>[2x]APRKFFVGGNWKMNGDKKSLGELIHTLNGAKLSADT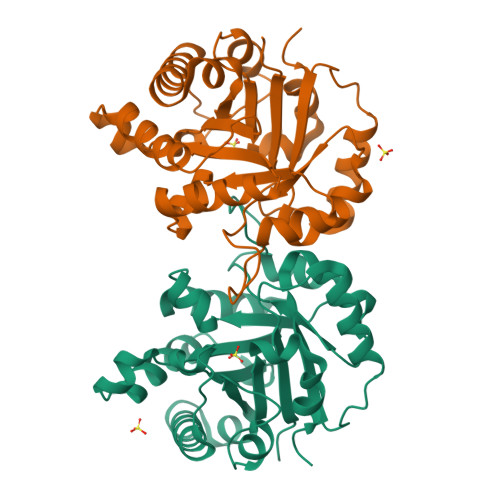EVVCGAPSIYLDFARQKLDAKIGVAAQNCYKVPKGAFTGEISPAMIKDIGAAWVILGHSERRHVFGESDELIGQKVAHALAEGLGVIACIGEKLDEREAGITEKVVFEQTKAIADNVKDWSKVVLAYEPVWAIGTGYSLTPQQAQEVHEKLRGWLKSHVSDAVAQSTRIIYGGSVTGGNCKELASQHDVDGFLVGGASLKPEFVDIINAKH>SGQRPSLPMLATDERSTDKESPNEDREFVPCSSLDVRRIYPKGPLLVLPEKIYLYSEPTVKELLPFD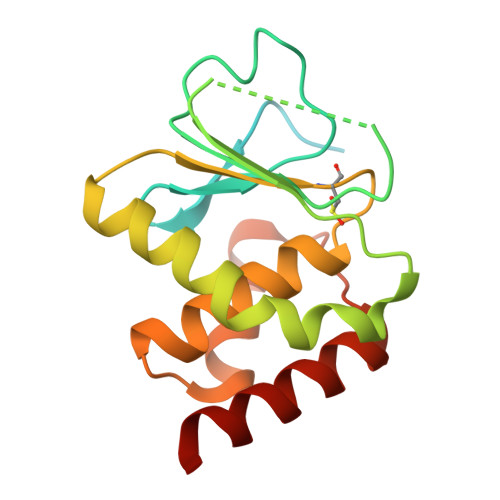VVINVAEEANDLRMQVPAVEYHHYRWEHDSQIALDLPSLTSIIHAATTKREKILIHCQCGLSRSATLIIAYIMKYHNLSLRHSYDLLKSRADKINPSIGLIFQLMEWEVALNAKT[2x]(5E,13E)-11-HYDROXY-9,15-DIOXOPROSTA-5,13-DIEN-1-OIC ACID | 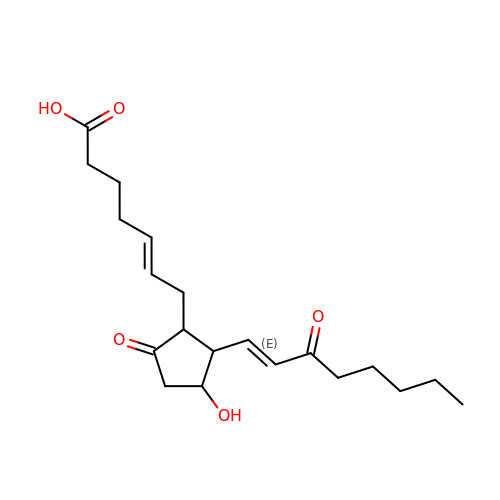C20 H30 O5 | YRTJDWROBKPZNV-SFTOQRQMSA-N>[2x]HNKVRTCWNEGRPALAGWLQLPGTLHAEALARLDYDAVVIDMQHSPIDFGQVAPMLIAIELGGAEPFVRTQVNDPSDIMKLLDAGAYGIIAPMVNTRAEAQTLASALHYSPRGLRAFGPRRPSLRYGSGYLAQAS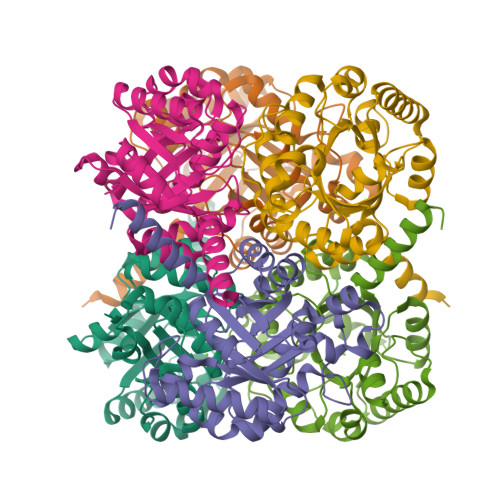ETVVGLAMIETREALANIDEILSVDGIDGVFIGPTDLALDLGHAPLVDTEEAEVVSAIAHVRERAHAAGKRVGIFCGSGGFARVKLAEGFDFVTAAPDLAMLSAAARQVIADARAL>[2x]YTPPGRLGDESSGPRTDPRFSPAMVEALATFGLDAVAAAPPVSASDDLPTVLAAVGASHDGFQAVYDSIALDL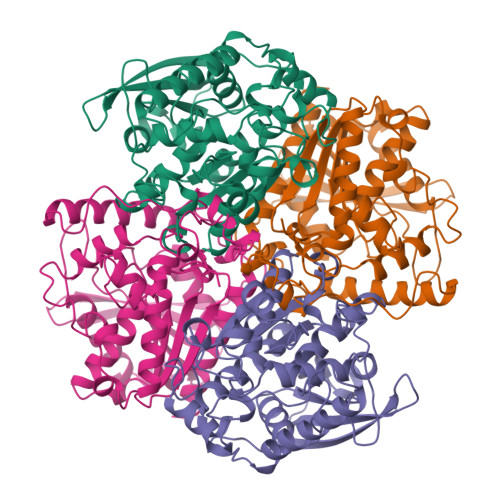PTDRDDVETSTETILGVDGNEITLHVFRPAGVEGVLPGLVYTHGGGMTILTTDNRVHRRWCTDLAAAGSVVVMVDFRNAWTAEGHHPFPSGVEDCLAAVLWVDEHRESLGLSGVVVQGESGGGNLAIATTLLAKRRGRLDAIDGVYASIPYISGGYAWDHERRLTELPSLVENDGYFIENGGMALLVRAYDPTGEHAEDPIAWPYFASEDELRGLPPFVVAVNELDPLRDEGIAFARRLARAGVDVAARVNIGLVHGADVIFRHWLPAALESTVRDVAGFAADRARLR N-[(S)-(biphenyl-4-ylmethoxy)(hydroxy)phosphoryl]-L-glutamic acid | 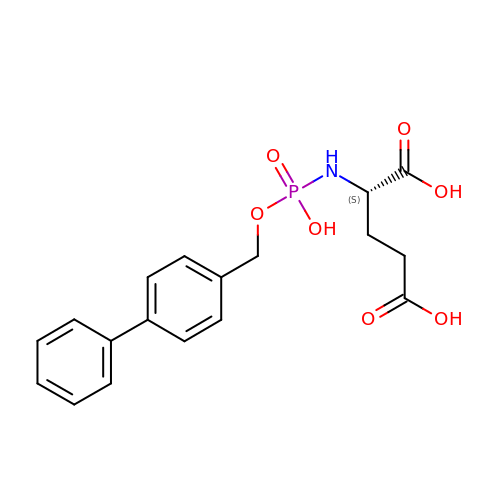C18 H20 N O7 P | DATQTWKKBHKLSV-INIZCTEOSA-N> SRLDPDPEFIGFINN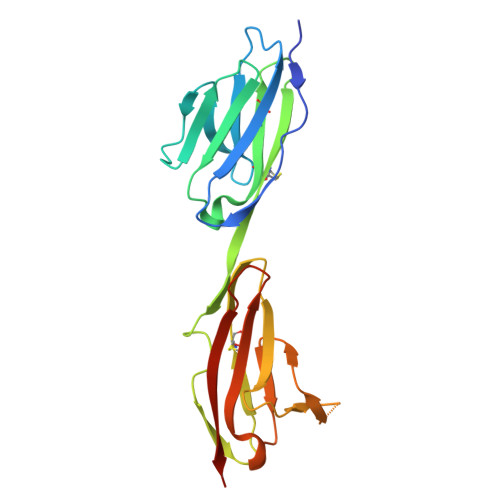VTYPAGREAILACSVRNLGKNKVGWLRASDQTVLALQGRVVTHNARISVMHQDMHTWKLKISKLRESDRGCYMCQINTSPMKKQVGCIDVQVPPDIINEESSADLAVQEGEDATLTCKATGNPQPRVTWRREDGEMILIRKPGSRELMKVESYNGSSLRLLRLERRQMGAYLCIASNDVPPAVSKRVSLSVHHHHHHH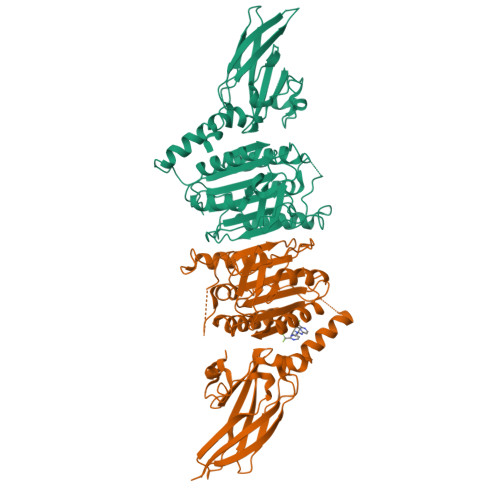>[2x]MLAKDKVALLIGNMNYREHPKLKAPLVDVYELTNLLRQLDFKVVSLLDLTEYEMRNAVDEFLLLLDKGVYGLLYYAGHGYENFGNSFMVPVDAPNPYRSENCLCVQNILKLMQEKETGLNVFLLDMCRKRNDYDDTIPILDALKVTANIVFGYATCQGAEAFEIQHSGLANGIFMKFLKDRLLEDKKITVLLDEVAEDMGKCHLTKGKQALEIRSSLSEKRALTDPIQGTEYSAESLVRNLQWAKAHELPESMCLKFKCGVQIQLGFAAEFSNVMIIYTKIVYKPPEIIMCDAYVTDFPLDLDIDPKDANKGTPEETGSYLVSKDLPKACLYTRLSSLQKLKEELVFTVCLSYQYSGLEDTVEDKQEVNVGKPLIAKLDMHRHHHHHH> GSTYDALRRQLIPSFDLLYGSAVSVVAMSVPATARILDLGAGTGLLGAALRERLPDAELLLQDRSQAMLEQARQRFADDDQVAIRVADHLDELPAGPFDAVVSALSIHALEHQDKQDLFTRIRKILRPGGIFVNVEQVLAPTSELEKMYDRQHEAHVLASDTPAEEWAAGRERMKHDIPIDVETQIQWLRDAGFTTADCLAKDWRFATYAGWNGS

Here, we characterize the O-methyltransferases BelI and CysG, which catalyze the initial step of β-lactone formation. Employing techniques such as crystallography, computational analysis, mutagenesis, and activity assays, we identified a His-His-Asp (HHD) motif in the active sites of the two enzymes, which is crucial for binding a catalytically active calcium ion. As expected, BelI as well as CysGΔN16 adopt the class I methyltransferase Rossmann fold, characterized by a core domain of a seven-stranded β-sheet flanked by α-helices. The HHD-motif enables regiospecific C1-carboxy group methylation of their respective malic substrates.

Due to the high crystallization tendency of CysGΔN16, subsequent mutagenesis experiments were focused on this variant. This approach enabled the production of both full-length and N-terminal truncated mutants in high purity, which were characterized in activity assays and used for structural studies. Therefore, we conducted structure-based mutagenesis by introducing non-conservative alanine residues in the HHD motif to further explore the metal-binding site.Nuclear-encoded pentatricopeptide repeat (PPR) proteins with a C-terminal DYW domain have been characterized as site-specific factors for C-to-U RNA editing in plant mitochondria and plastids. Here we report crystal structures of the DYW domain of an Arabidopsis thaliana (A. thaliana) plastid RNA editing factor, OTP86, as the outcome of a solubility and crystallization screening of over 100 different DYW domain constructs from 30 PPR proteins. OTP86 was characterized as a site-specific factor for an editing site in rps14 transcripts. Herein we describe structures of a DYW domain and find that, apart from a cytidine deaminase fold, DYW domains contain a characteristic DYW motif, stabilized by a zinc atom, as well as a gating domain that controls zinc-mediated catalysis sterically and catalytically.

Finally, we obtained crystals of OTP86DYW belonging to space group C2 and diffracting to a resolution of 2.5 Å. The structure was solved by single-wavelength anomalous dispersion (SAD) phasing harnessing four zinc atoms (c for details). Remarkably, the deaminase fold of OTP86DYW is interrupted by an insertion of about 55 residues that bridge β-strand 2 and α-helix 2. We conclude that the OTP86DYW active site seems to have limited accessibility for sub-strate cytidines, which is conferred by an insertion (H837-G891), and we thus term this insertion gating domain. In OTP86DYW, the motif terminates with the DSW sequence and provides two ligands (C954, C956) for a second zinc ion (Zn2); two more ligands are part of the deaminase domain (H924 and H947), indicating that Zn2 only has a structural role within DYW domains. Notably, the surface charge distribution of OTP86DYW reveals a region of positively charged residues spanning across the active site and passing in between the base of the gating domain’s β-finger and the DYW motif. The inactive structure zinc coordination is maintained by coordinating H892, C920, C923 and a more distant water molecule, whereas the catalytically important E894 is ionically bonded to K915; K915 also hydrogen bonds to S828 and S893. In this configuration, the ion pair will reduce the basic character of E894 and hinder the required deprotonation of the deaminating water, which is not productively coordinated by Zn1 and also not contacted by E894. We reason that beyond the steric inhibition through the gating domain, K915 has to be released before efficient catalysis can occur. For example, the cytidine bound to MmCD causes steric clashes with the β-finger of the OTP86DYW gating domain when positioned in the active site of OTP86DYW.

>[2x]GAMGCSWIEMDGKVHKFTARDKSHPESKEIYEKLSEVTRKLEREVGYVADTKFVLHNVDEGEKVQMLHGHSERIAIAYGLLRTPDRACLRITKNLRVCRDCHTFCKLVSKLFRRDIVMRDANRFHHFESGLCSCGDSW>[6x]MSEEDKAKKLENLLKLLQLNNDDTSKFTQEQKKAMKDHKFWRTQPVKDFDEKVVEEGPIDKPKTPEDISDKPLPLLSSFEWCSIDVDNKKQLEDVFVLLN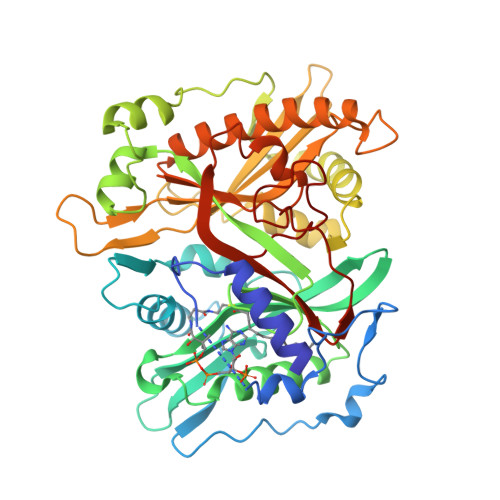ENYVEDRDAGFRFNYTKEFFNWALKSPGWKKDWHIGVRVKETQKLVAFISAIPVTLGVRGKQVPSVEINFLCVHKQLRSKRLTPVLIKEITRRVNKCDIWHALYTAGIVLPAPVSTCRYTHRPLNWKKLYEVDFTGLPDGHTEEDMIAENALPAKTKTAGLRKLKKEDIDQVFELFKRYQSRFELIQIFTKEEFEHNFIGEESLPLDKQVIFSYVVEQPDGKITDFFSFYSLPFTILNNTKYKDLGIGYLYYYATDADFQFKDRFDPKATKALKTRLCELIYDACILAKNANMDVFNALTSQDNTLFLDDLKFGPGDGFLNFYLFNYRAKPITGGLNPDNSNDIKRRSNVGVVML>GCAUCCG[2x];>[2x]CGGA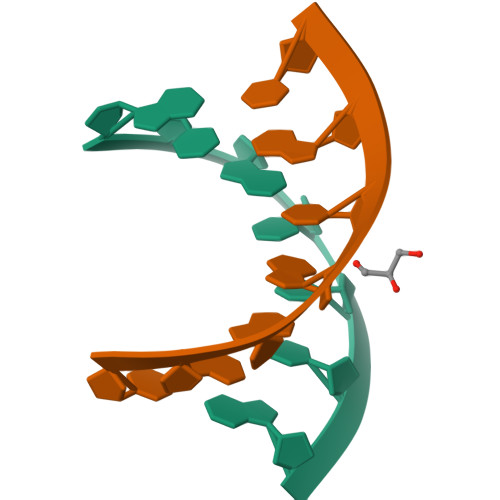UGC>[2x]GSHMASMKPIFDINETFEKQLKDLTSNVKSIQDNLLEEIITPNTKTEYLQRFLIDRFDKELFKKNVPIVSYEDIKPYLDRVVNGESSDVISARTITGFLLSSGTSGGAQKMMPWNNKYLDNLTFIYDLRMQVITKHVKGVEEGKGMMF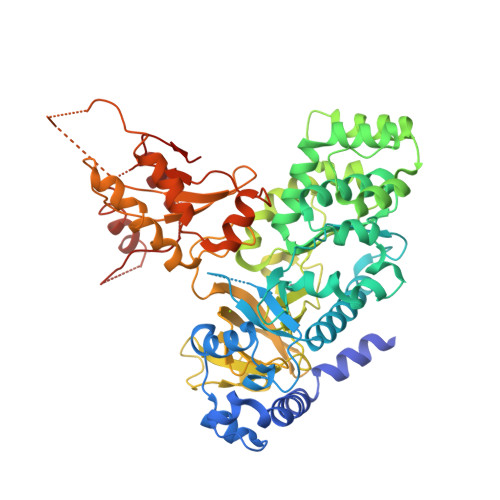LFTKQESMTPSGLPARVATSSYFKSDYFKNRPSNWYYSYTSPDEVILCPNNTESLYCHLLCGLVQRDEVVRTGSIFASVMVRAIEVLKNSWEELCSNIRSGHLSNWVTDLGCQNSVSLVLGGPRPELADTIEEICNQNSWKGIVKRLWPNTKYIETVVTGSMGQYVPMLNYYCNDLPLVSTTYGSSETTFGINLDPLCKPEDVSYTFMPNMSYFEFIPMDGGDKNDVVDLEDVKLGCTYEPVVTNFAGLYRMRVGDIVLVTGFYNNAPQFKFVRRENVVLSIDSDKTNEEDLFKAVSQAKLVLESSGLDLKDFTSYADTSTFPGHYVVYLEVDTKEGEEKETAQFELDEEALSTCCLVMEESLDNVYKRCRFKDGSIGPLEIRVVRQGTFDSLMDFFISQGASTGQYKTPRCIKSGKALQVLETCVVAKFFSI> MNRDIGKNAERELVSILRGEGFN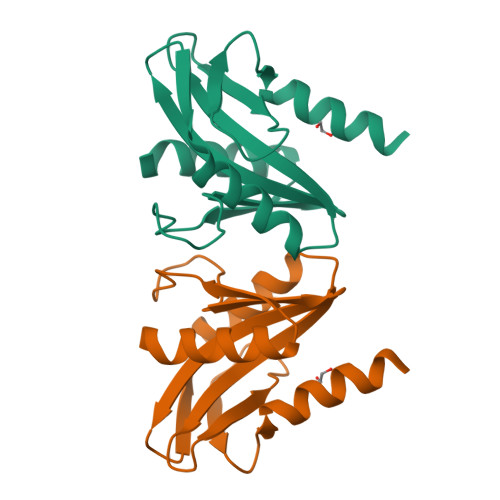AVRIPTSNSSPNPLPDIFATKGNTLLSIECKSTWENKVKVKEHQVRKLLDFLSMFTMKGVPLIAIKFKQVHEWRVLVPEKAEDIIVTIDNSIPIEDLFKILEKRIEEKILTP>GPGVDEALREAQTKSAMNFIKDNSRALIQRMGMTVIKQITDDLFVWNVLNREEVNIICCEKVEQDAARGIIHMILKKGSESCNLFLKSLKEWNYPLFQDLN[12x]

Many NLR proteins nucleate the “inflammasome”—a large macromolecular complex that triggers inflammatory cell death and cytokine secretion in response to microbial or danger-associated ligands. Like many other supramolecular assemblies in the human innate immune system, the inflammasome complex relies on homotypic and heterotypic interactions between the death domains (DDs) to initiate, amplify, and propagate pyroptotic signaling. Inflammasome sensor NLRs can be grouped into two categories based on their DDs: PYRIN domain (PYD) and caspase activation and recruitment domain (CARD), both domains were found to form filamentous complexes to initiate the inflammasome formation. Extending this analysis, we also found that specific type II interface motifs directly dictate the compatibility of heterotypic pairwise CARD-CARD interactions among NLRP1, CARD8, NLRC4, ASC, and CASP1.

To extend these results beyond NLRP1 and CARD8 and test the predictive power of our model, we examined a third CARD-containing NLR sensor, NLRC4. To unambiguously assign the Type II interface residues of human NLRC4-CARD, we determined its filament structure at 3.3 Å using cryo-EM. The final polished structure closely agrees with previously published findings. Interestingly, unlike NLRP1-CARD and CARD8-CARD, the strong density bridge in the Type II interface is absent within NLRC4-CARD filaments. The Type IIb tyrosine residue (Tyr78) is folded backward toward the hydrophobic core and does not participate in intermolecular Type II interaction. Instead, two nearby small residues, Asn77 and Gln82, come forward to form a class of Type II junction that is more flexible than that of NLRP1 and CARD8. Molecular docking predicted that NLRC4 Type IIb surface would be structurally compatible with both ASC-CARD and CASP1-CARD. This was validated using the in vitro EMSA assay (lanes 6–7 in both panels) and in 293 T cells. Overexpressed NLRC4-CARD nucleated the formation of both ASC-GFP and CASP1 C285G-GFP specks, as well as ASC-CARD-GFP and CASP1-CARD-GFP filaments at similar levels. The versatility of human NLRC4-CARD is in agreement with previous studies on murine Nlrc4.>SQAEFDKAAEEVKHLKTKPADEEMLFIYSHYKQATVGDINTERPGMLDFKGKAKWDAWNELKGTSKEDAM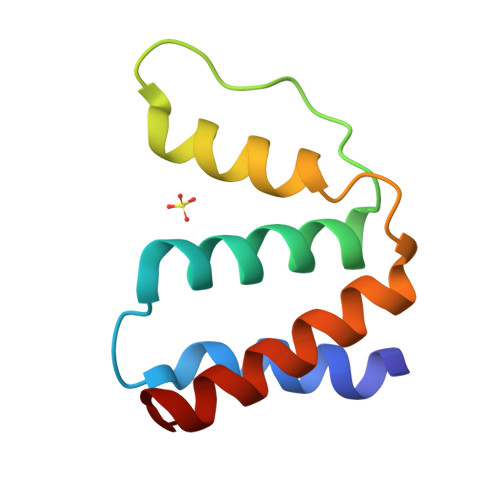KAYIDKVEELKKKYGI[3x]>[5x]ME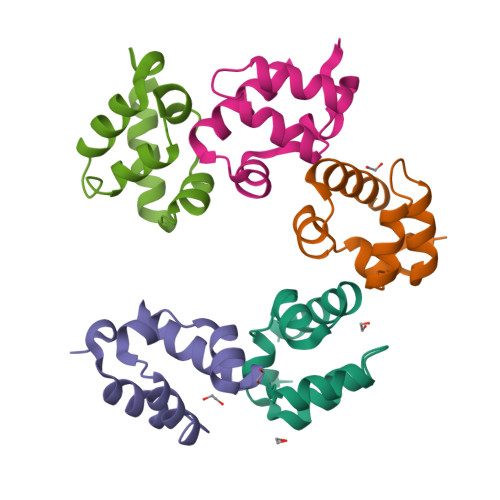KTRTEPSIWTVDDVWAFIHSLPGCQDIADEFRAQEIDGQALLLLKEDHLMSAMNIKLGPAEKICARINSLKESRHHHHHH>[2x]MMMTGTIETTGNISAEKGGSIILQCHLSSTTAQVTQVNWEQQDQLLAICNADLGWH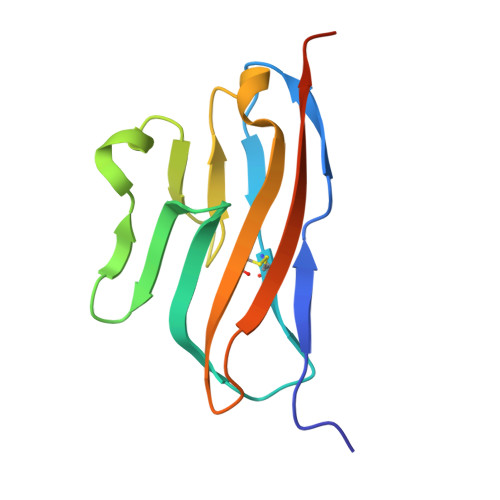ISPSFKDRVAPGPGLGLTLQSLTVNDTGEYFCIYHTYPDGTYTGRIFLEVLESSVAEHGAR>[3x]MKIATITGVTKSPELQVTKAIGALILSSDVALSALTTEKISIYIERGNGSNVILANKVLL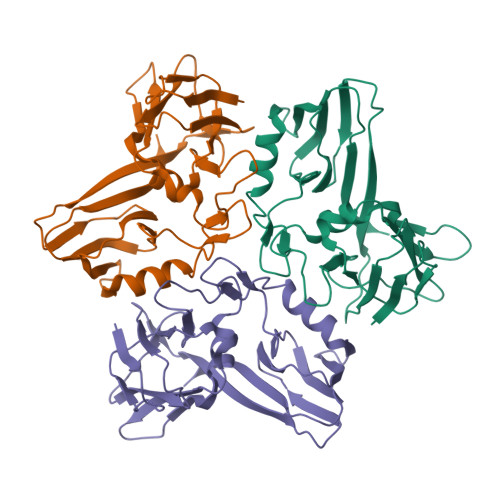KDFILASTYGTENTQSDADNAMIALCELADEGSIYLADKESIKITLEDLISDKRYDLHGIEEPQQTNNLFFFEQKSVASEEFNKKIDVQGFDLAIMTVDDSVSDLSYQYSNGQVVKYLPFELQTLSRDIDPIQAVLSDGKVVQGLTDRLTLPLVAVVGIEINKSQGSIINFVVRCLKTV ABCG2 is an ABC transporter of broad substrate specificity expressed in various tissues and tissue barriers. ABCG2 also functions as a multidrug transporter and exports a wide range of xenobiotics and pharmaceuticals, thus strongly impacting their pharmacokinetics. Here we present cryo-EM structures of ABCG2 under turnover conditions containing either the endogenous substrate estrone-3-sulfate or the exogenous substrate topotecan. We find two distinct conformational states in which both the transport substrates and ATP are bound.

In contrast, the turnover sample containing topotecan revealed two well-ordered structures, which we termed turnover-1 and turnover-2 states, resolved at 3.1 Å and 3.4 Å, respectively. In the topotecan-bound ABCG2 sample, the dominant class (88% of the ordered particles) belonged to the turnover-1 state, whereas 12% particles belonged to the turnover-2 state. Whereas the state turnover-1 features more widely separated NBDs and an accessible substrate cavity between the TMDs, turnover-2 features semi-closed NBDs and an almost fully occluded substrate cavity. In turnover-2, the topotecan density was narrower in the horizontal dimension and longer in the vertical dimension, probably reflecting a rotation of the drug compared to the turnover-1 state. In turnover-2, the gap is even smaller, causing the entrance to cavity 1 from within the membrane to be completely sealed and even the opening to the cytosol to be reduced. In turnover-2, the distance between the coupling helices is reduced by another 4.0 Å. We now found that in turnover-2, Q181 and F182 facilitated contacts between TM1 of one ABCG2 monomer and TM5’ of the other, thus helping stabilize the TMD domain closure. In addition, the arginine residue R184 provides a direct contact, in the form of a cation-π interaction, with the adenine moiety of the ATP molecule bound to the opposite NBD. In contrast, the R482 side chain is rotated towards the external side of the membrane in turnover-2, where the guanidinium group contacts side chains and main-chain atoms from TM2 and TM4 in the direct vicinity of F439 (right). The concerted motions of TM1, TM2, and TM5 reduce the volume of cavity 1 by approximately one-third, from ~1300 Å3 in turnover-1 to ~830 Å3 in turnover-244, which is incompatible with the binding of the inhibitor molecules.

>MDYKDDDDKGSSSSNVEVFIPVSQGNTNGFPATASNDLKAFTEGAVLSFHNICYRVKLKSGFLPCRKPVEKEILSNINGIMKPGLNAILGPTGGGKSSLLDVLAARKDPSGLSGDVLINGAPRPANFKCNSGYVVQDDVVMGTLTVRENLQFSAALRLATTMTNHEKNERINRVIQELGLDKVADSKVGTQFIRGVSGGERKRTSIGMELITDPSILFLDEPTTGLDSSTANAVLLLLKRMSKQGRTIIFSIHQPRYSIFKLFDSLTLLASGRLMFHGPAQEALGYFESAGYHCEAYNNPADFFLDIINGDSTAVALNREEDFKATEIIEPSKQDKPLIEKLAEIYVNSSFYKETKAELHQLSGGEKKKKITVFKEISYTTSFCHQLRWVSKRSFKNLLGNPQASIAQIIVTVVLGLVIGAIYFGLKNDSTGIQNRAGVLFFLTTNQCFSSVSAVELFVVEKKLFIHEYISGYYRVSSYFLGKLLSDLLPMRMLPSIIFTCIVYFMLGLKPKADAFFVMMFTLMMVAYSASSMALAIAAGQSVVSVATLLMTICFVFMMIFSGLLVNLTTIASWLSWLQYFSIPRYGFTALQHNEFLGQNFCPGLNATGNNPCNYATCTGEEYLVKQGIDLSPWGLWKNHVALACMIVIFLTIAYLKLLFLKKYS[2x]>MKIVIVKKVEIQVAGRTGMRCASSCGAKS[2x];> MRIGFNFTLGETLPLVRQLAQEGAIDYCELLIDNFMQVPPQELAEAFDVPVGFHIMFSRFIESDEEQLRDFAARLRPYIEALRPLYVSDHIAYFSHQGRALYHLGEIDYAADYERVRARAALWQSLLGQTIHFENYPSIVDGGHAAPAFFQRLARDTGAGVLFDVSNAVCAWRNDGPEVAAWRGVMAGASHFHVGGYAGAFIDEGVTVDTHDRALAQDTLDSLRRHRDVLDKPGATITYERDENIDIDGVRADLLALRAIFPR;>[2x]MNAPTTAAAGAAPGRQVKDSELLARLADPAARGDFPPGCRAHVRIDISIRAYWHTLFDICPGLLDIADPDGMAIFAPFMDWARRENLTMGWSFYIWVGRWLAQSPWRERLDEELTQALLSASAARWAVLDRSADVGVVLGRRGSDDWIIGWKPNTLAAGRRVELVSLDGQLPRPAEDVGVFHLAGYELDSFPGWLALPR;> MRIGFNFTLGETLPLVRQLAQEGAIDYCELLIDNFMQVPPQELAEAFDVPVGFHIMFSRFIESDEEQLRDFAARLRPYIEALRPLYVSDHIAYFSHQGRALYHLGEIDYAADYERV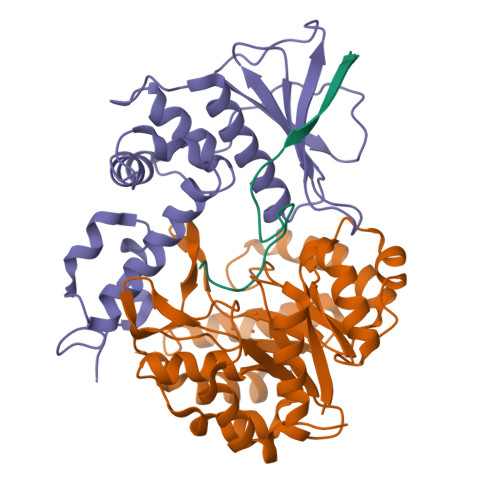RARAALWQSLLGQTIHFENYPSIVDGGHAAPAFFQRLARDTGAGVLFDVSNAVCAWRNDGPEVAAWRGVMAGASHFHVGGYAGAFIDEGVTVDTHDRALAQDTLDSLRRHRDVLDKPGATITYERDENIDIDGVRADLLALRAIFPRG>[3x]SNAMANTSSDWAGAPQNASADGEFVRDTNYIDDRIVADVPAGSEPIAQEDGTFHWPVEAGRYRLVAARACPWAHRTVITRRLLGLENVISLGLTGPTHDVRS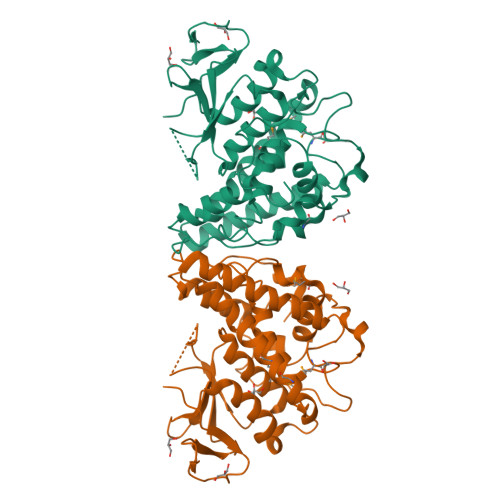WTFDLDPNHLDPVLQIPRLQDAYFNRFPDYPRGITVPALVEESSKKVVTNDYPSITIDFNLEWKQFHREGAPNLYPAELREEMAPVMKRIFTEVNNGVYRTGFAGSQEAHNEAYKRLWVALDWLEDRLSTRRYLMGDHITEADIRLYPTLVRFDAVYHGHFKCGRNKITEMPNLWGYLRDLFQTPGFGDTTDFTEIKQHYYITHAEINPTRIVPVGPDLSGFATPHGREKLGGSPFAEGVTLPGPIPAGEEVKNPEPFQK>HMEPKVGVIYGLAVLGAGGIGDVTKIIVQILESKNPGTHLLNISGDIAKHSITLASALSKKLVAEKKLPLPKKDIDLNNKEIYIQFSQSYSKIDGDSATAAVCLAIISALLDIPLKQDFAITGSLDLSGNVLAIGGVNEKIEAA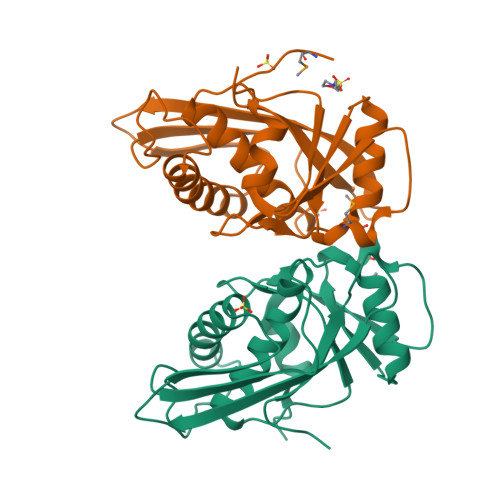KRYGFKRVIIPEANMIDVIETEGIEIIPVKTLDEIVPLVFDLD[2x]> MTTIVSVRRNGHVVIAGDGQATLGNTVMKGNVKKVRRLYNDKVI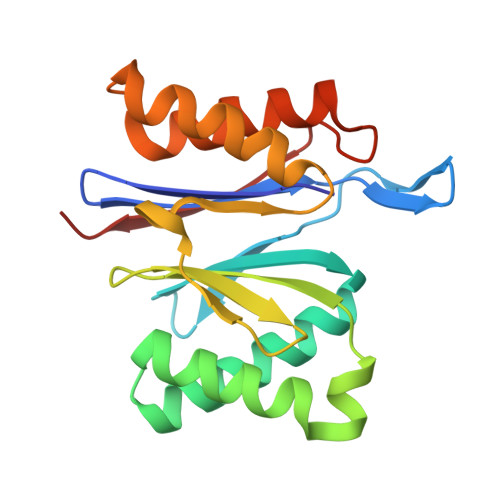AGFAGGTADAFTLFELFERKLEMHQGHLVKAAVELAKDWRTDRMLRKLEALLAVADETASLIITGNGDVVQPENDLIAIGSGGPYAQAAARALLENTELSAREIAEKALDIAGDICIYTNHFHTIEELSYKA> MMRRLALQSSIRRATPFATPLVASTKALNPMCSAITIREASTVAISVQGLHYVGTGLAAIALAGVGLGIGTIFGNLLVACARQPNLTKMLFNYAILG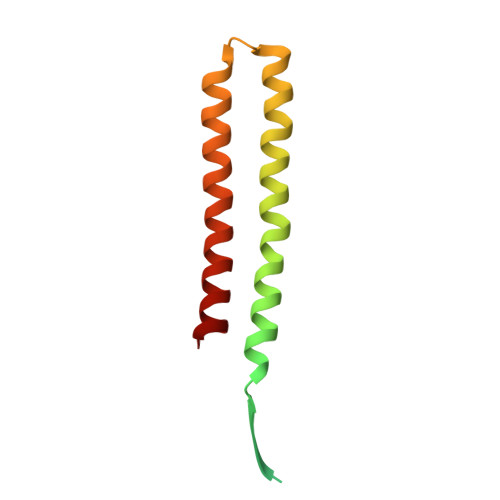FALTEAIGLFALMLAFLMLFS>MLSPQRVAAAASRGADDAMESSKPGPVQVVLVQKDQHSFELDEKALASILLQDHIRDLDVVVVSVAGAFRKGKSFILDFMLRYLYSQKESGHSNWLGDPEEPLTGFSWRGGSDPETTGIQIWSEVFTVEKPGGKKVAVVLMDTQGAFDSQSTVKDCATIFALSTMTSSVQIYNLSQNIQEDDLQQLQLFTEYGRLAMDEIFQKPFQTLMFLVRDWSFPYEYSYGLQGGMAFLDKRLQVKEHQHEEIQNVRNHIHSCFSDVTCFLLPHPGLQVATSPDFDGKLKDIAGEFKEQLQALIPYVLNPSKLMEKEIN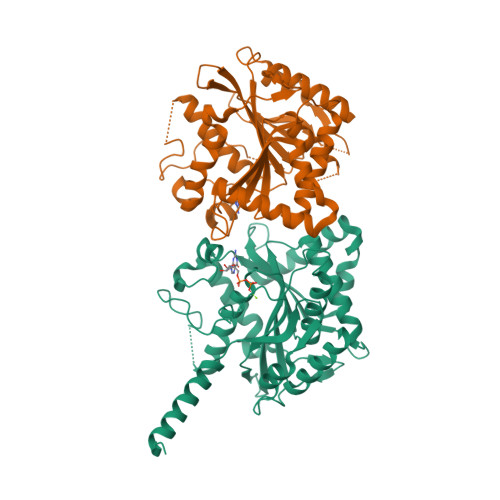GSKVTCRGLLEYFKAYIKIYQG[2x]>[4x]MTESQSYETRQARPAGQSLAERVARLVAIDPQAAAAVPDKAVAERATQQGLRLAQRIEAFLSGYGDRPALAQRAFEITKDPITGRAVATLLPKFETVSYRELLERSHAIASELANHAEAPVKAGEFIATIGFTSTDYTSLDIAGVLLGLTSVPLQTGATTDTLKAIAEETAPAVFGASVEHLDNAVTTALATPSVRRLLVFDYRQGVDEDREAVEAARSRLAEAGSAVLVDTLDEVIARGRALPRVALPPATDAGDDSLSLLIYTSGSTGTPKGAMYPERNVAQFWGGIWHNAFDDGDSAPDVPDIMVNFMPLSHVAGRIGLMGTLSSGGTTYFIAKSDLSTFFEDYSLARPTKLFFVPRICEMIYQHYQSELDRIGAADGSPQAEAIKTELREKLLGGRVLTAGSGSAPMSPELTAFIESVLQVHLVDGYGSTEAGPVWRDRKLVKPPVTEHKLIDVPELGYFSTDSPYPRGELAIKT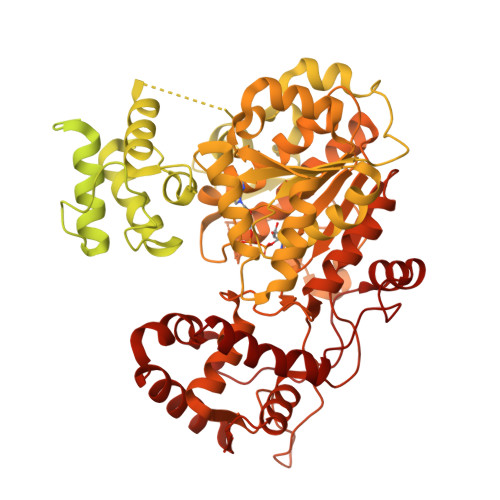QTILPGYYKRPETTAEVFDEDGFYLTGDVVAEVAPEEFVYVDRRKNVLKLSQGEFVALSKLEAAYGTSPLVRQISVYGSSQRSYLLAVVVPTPEALAKYGDGEAVKSALGDSLQKIAREEGLQSYEVPRDFIIETDPFTIENGILSDAGKTLRPKVKARYGERLEALYAQLAETQAGELRSIRVGAGERPVIETVQRAAAALLGASAAEVDPEAHFSDLGGDSLSALTYSNFLHEIFQVEVPVSVIVSAANNLRSVAAHIEKERSSGSDRPTFASVHGAGATTIRASDLKLEKFLDAQTLAAAPSLPRPASEVRTVLLTGSNGWLGRFLALAWLERLVPQGGKVVVIVRGKDDKAAKARLDSVFESGDPALLAHYEDLADKGLEVLAGDFSDADLGLRKADWDRLADEVDLIVHSGALVNHVLPYSQLFGPNVVGTAEVAKLALTKRLKPVTYLSTVAVAVGVEPSAFEEDGDIRDVSAVRSIDEGYANGYGNSKWAGEVLLREAYEHAGLPVRVFRSDMILAHRKYTGQLNVPDQFTRLILSLLATGIAPKSFYQLDATGGRQRAHYDGIPVDFTAEAITTLGLAGSDGYHSFDVFNPHHDGVGLDEFVDWLVEAGHPISRVDDYAEWLSRFETSLRGLPEAQRQHSVLPLLHAFAQPAPAIDGSPFQTKNFQSSVQEAKVGAEHDIPHLDKALIVKYAEDIKQLGLL>MGIKLKRLSDKPVLMPKAENEWERAAVFNTAAIYDNGLFHLIYRATDIGPHAKYGKYISRLGYAVSKDGINFMRLDKPVMSNETEQELRGLEDPRIVKIDGIYYMMYTGFGDRFQDDYRICLATSKNLIDWERKGVVLDEPNKDASLFPEKINGKYVMLHRRYPDIWIAFSDDLKNWYDHKPILKPIPNTWESARVGIGGPPIKTKDGWFLIYHAADDNNVYRLGAVLLDLEDPSKVIARQKEPILEPELGWEKEGYIPNVVFSCGNAVKDDTIYVYYGGADTVIGVA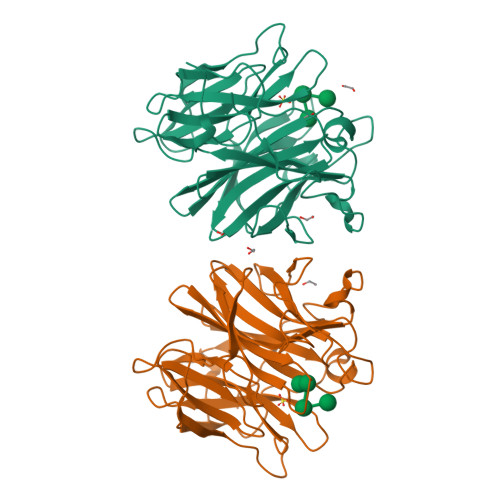ILEMKDIKFHHHHHH[2x]> MKSNEHDDCQVTNPSTGHLFDLSSLSGRAGFTAAYAKGWGVYMSICGENENCPPGVGACFGRTRISVGKANKRLRYVDQVLQLVYKDGSHCPSKHG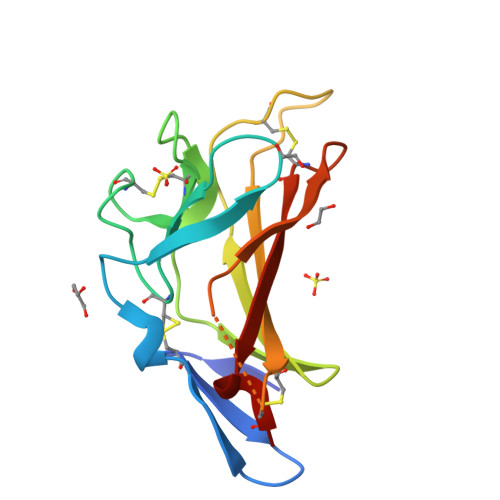LSYKSVISFVCRPEAGPTNRPMLISLDKQTCTLFFSWHTPLACELA>GMSAPEDWNSQVIQEFRANGGRVGGNFEGAPMVLVHHVGRKTGKAAVTPMMYLPSDDDPGTIYVFASKAGAASNPAWYYNLTTAGTAQVEVGTETYAVGVTEVTGEDRDRIYSEQARRYPGFADYEKKTAGIRTIPVLAL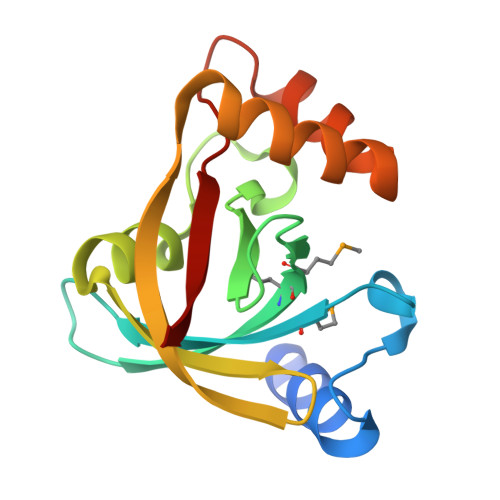TRT[4x]>MVLYFIGLGLYDERDITVKGLEIAKKCDYVFAEFYTSLMAGTTLGRIQKLIGKEIRVLSREDVELNFENIVLPLAKENDVAFLTPGDPLVATTHAELRIRAKRAGVESYVIHAPSIYSAV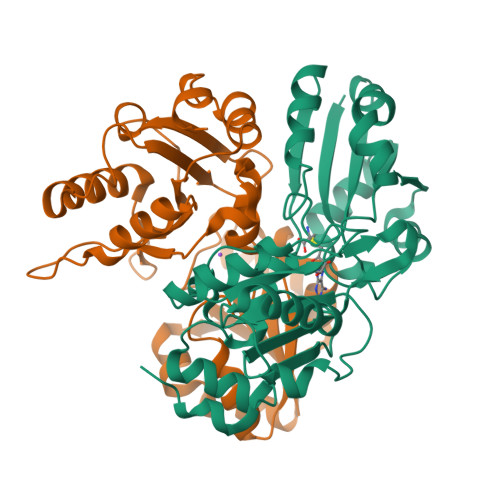GITGLHIYKFGKSATVAYPEGNWFPTSYYDVIKENAERGLHTLLFLDIKAEKRMYMTANEAMELLLKVEDMKKGGVFTDDTLVVVLARAGSLNPTIRAGYVKDLIREDFGDPPHILIVPGKMHIVEAEYLVEIAGAPREILRVNV[2x]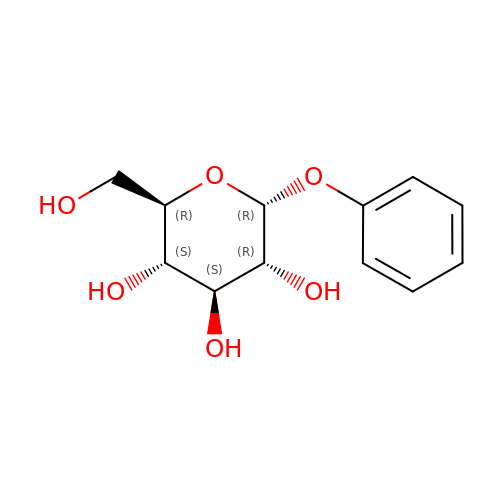(2R,3S,4S,5R,6R)-2-(hydroxymethyl)-6-phenoxy-oxane-3,4,5-triol | C12 H16 O6 | NEZJDVYDSZTRFS-ZIQFBCGOSA-N(3R)-1,2-oxazolidin-3-amine | C3 H8 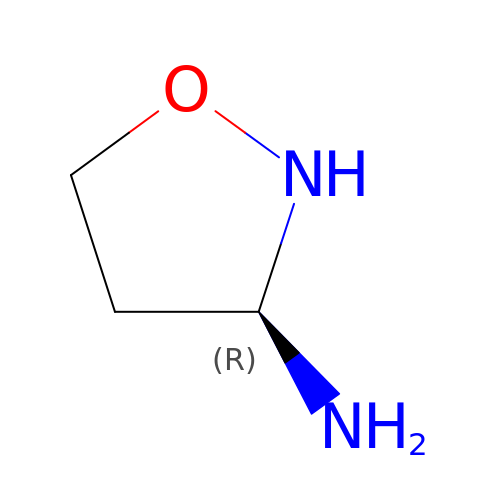N2 O | IRMAFFLFVPYKOZ-GSVOUGTGSA-N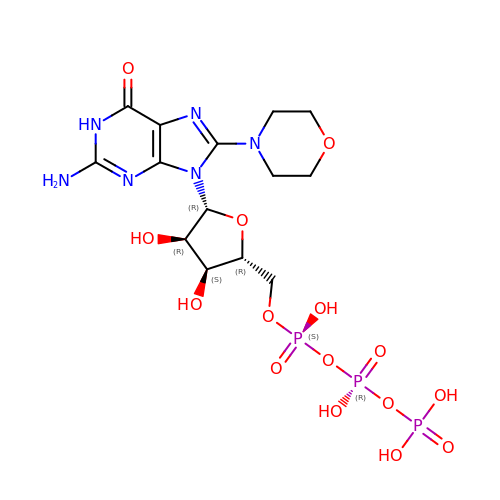8-morpholin-4-ylguanosine 5'-(tetrahydrogen triphosphate) | C14 H23 N6 O15 P3 | YYAPYNUGMUZNGD-WOUKDFQISA-N2-(2-chlorophenyl)sulfanyl-~{N}-[(4-cyanophenyl)methyl]-~{N}-[(5-methyl-1,3,4-oxadiazol-2-yl)methyl]ethanamide | C20 H17 Cl N4 O2 S 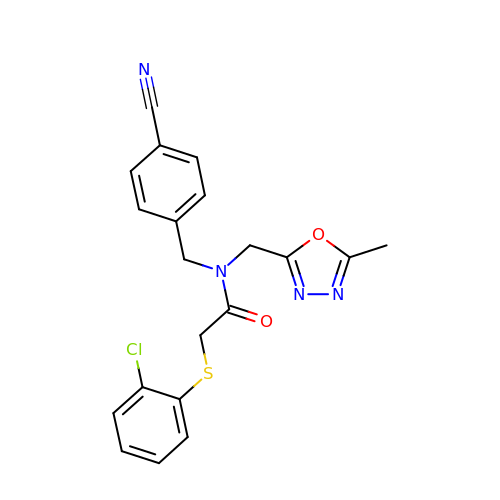| ZOCHVZHQWHVDHH-UHFFFAOYSA-N> MNTYAQESKLRLKTKIGADGRCVIEDNFFTPPFKLMAPFYPKDDLAEIMLLAVSPGMMRGDAQDVQLNIGPNCKLRITSQSFEKIHNTEDGFASRDMHIVVGENAFLDFAPFPLIPFENAHFKGNTTISLRSSSQL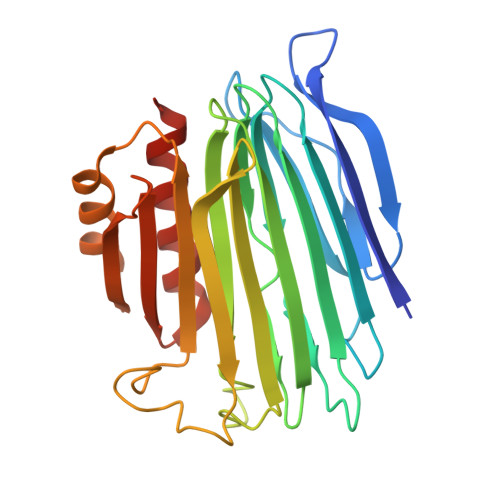LYSEIIVAGRVARNELFKFNRLHTKISILQDEKPIYYDNTILDPKTTDLNNMCMFDGYTHYLNLVLVNCPIELSGVRECIEESEGVDGAVSETASSHLCVKALAKGSEPLLHLREKIARLVTQTTTQKV>[4x]GSHMTDLAGPTITPNLQLVYVSNVERSTDFYRFIFKKEPVFVTPRYVAFPSSGDALFAIWSGGEEPVAEIPRFSEIGIMLPTGEDVDKLFNEWTKQKSHQI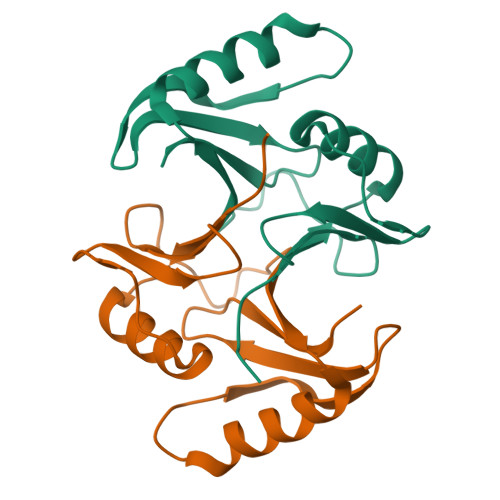IVIKEPYTDVFGRTFLISDPDGHIIRVCPLD>[7x]GAIFLEGVTVKGVTQVTTQPKLGEVQQKCHQFCGWEGSGFPGAQPVSMDKQNIKLLDLKPYKVSWKADGTRYMMLIDGTN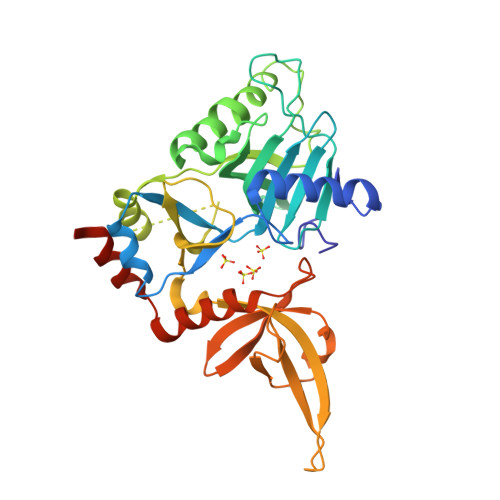EVFMIDRDNSVFHVSNLEFPFRKDLRMHLSNTLLDGEMIIDRVNGQAVPRYLIYDIIKFNSQPVGDCDFNVRLQCIEREIISPRHEKMKTGLIDKTQEPFSVRNKPFFDICTSRKLLEGNFAKEVSHEMDGLIFQPTGKYKPGRCDDILKWKPPSLNSVDFRLKITRMGGEGLLPQNVGLLYVGGYERPFAQIKVTKELKQYDNKIIECKFENNSWVFMRQRTDKSFPNAYNTAMAVCNSISNPVTKEMLFEFIDRCTALEHHHHHH> ETGVPEAFLLFSRRADIRRISLETNNNNVAIPLTGVKEASALDFDVTDNRIYWTDISLKTISRAFMNGSALEHVVEFGLDYPEGMAVDWLGKNLYWADTGTNRIEVSKLDGQHRQVLVWKDLDSPRALALDPAEGFMYWTEWGGKPKIDRAAMDGSERTTLVPNVGRANGLTIDYAKRRLYWTDLDTNLIESSNMLGLNREVIADDLPHPFGLTQYQDYIYWTDWSRRSIERANKTSGQNRTIIQGHLDYVMDILVFHSSRQSGWNECASSNGHCSHLCLAVPVGGFVCGCPAHYSLNADNRTCSAPTTFLLFSQKSAINRMVIDEQQSPDIILPIHSLRNVRAIDYDPLDKQLYWIDSRQNMIRKAQEDGSQGFTVVVSSVPSQNLEIQPYDLSIDIYSRYIYWTCEATNVINVTRLDGRSVGVVLKGEQDRPRAVVVNPEKGYMYFTNLQERSPKIERAALDGTEREVLFFSGLSKPIALALDSRLGKLFWADSDLRRIESSDLSGANRIVLEDSNILQ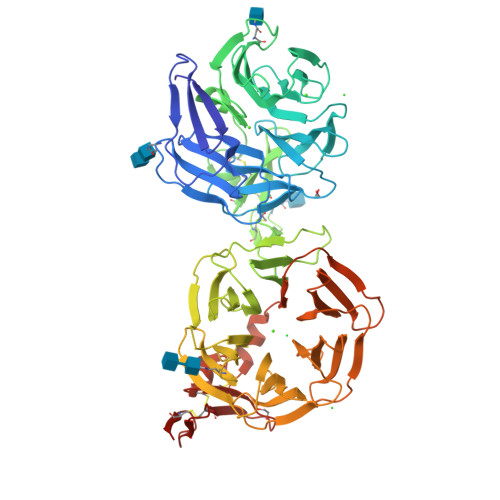PVGLTVFENWLYWIDKQQQMIEKIDMTGREGRTKVQARIAQLSDIHAVKELNLQEYRQHPCAQDNGGCSHICLVKGDGTTRCSCPMHLVLLQDELSCGGTKHHHHHH>[2x]MHHHHHHENLYFQSHMLLKPLQVYTADNQLIAEYGGKLSIPVEYKQIPPNFIHAFLAAEDSSFFEHSGISFKGLGRALSESVTGSDVQTGGSTITMQVAKNYYLSPERTLKRKITEIFLARKIEQNLSKEDILSLYVNKIFLGKNAYGIAAAAKIYYNKSINELSIAQMAMIAGLPKAPSKYNPVVNPERALERRNWILGRMLQLGYISQAEYQKAVAEPINLNMPNRDLNNIHPYAGEMVRSELVKHFGEQAIDSGYKVYTTINAKRQAIAEKAVQDGLEAYDRRHGWRGAEAHDKPLSEFRAYANTYPAQVTKVNSSSFEALMQDGSTVTVQWSGMSWARPYRNANSVGAAPSRASQIVKVKDIVRLRPNEAKTAWSLVQVPKVQGQLIAINPNDGSIEAIVGGYNFYQSKFNRALQGWRQPGSTIKPFLYALALERGMTPYSMVNDSPITIGKWTPKNSDGRYLGMIPLRRALYLSRNTVSVRLLQT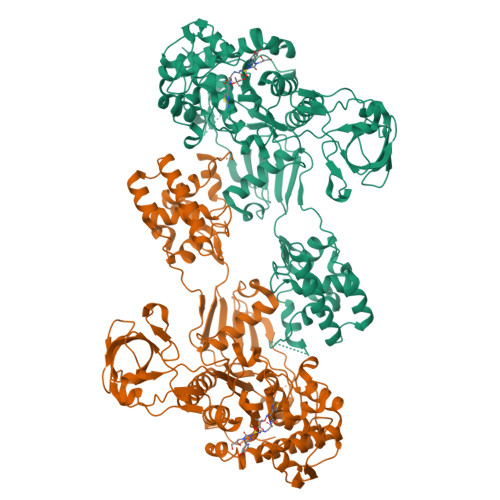VGIERTRQLFMDFGLQEDQIPRNYTIALGTPQVLPIQMATGYATFANGGYRVQPHFIQRIEDAYGKVIYEAKPEYACIPCINAPETTDDAQVTTPDDQVVEVTNKELEQKEKTTKQLNLKQTDKNNSQYRQAQRILKSSSAYDMANILRDVIEHGTGRAALKIGRSDLGGKTGTTNDAKDAWFAGFNGKLVTVTWVGFDQPTTLGRREYGGIAALPIWINFMGQALQGTPAAWVRLEKDAQ Most Gram-negative bacteria synthesize osmo-regulated periplasmic glucans (OPG) in the periplasm or extracellular space. In this study, structural and functional analyses of OpgG and OpgD from Escherichia coli revealed that these proteins are β-1,2-glucanases with remarkably different activity from each other, establishing a new glycoside hydrolase family, GH186. Furthermore, a reaction mechanism with an unprecedentedly long proton transfer pathway among glycoside hydrolase families is proposed for OpgD. The conformation of the region that forms the reaction pathway differs noticeably between OpgG and OpgD, which explains the observed low activity of OpgG.

The D388N mutant was used to determine a Michaelis complex structure of EcOpgD because this mutant displayed the lowest activity among mutants of acidic amino acids conserved in its homologs, and this residue is located in the long cleft of the ligand-free structure. The complex structure was obtained as a dimer by co-crystallizing the D388N mutant with β-1,2-glucan. The substrate binding site is formed as a cleft in the ligand-free structure, whereas this site forms a tunnel in the structure of the complex. In EcOpgD, the seventh and eleventh Glc moieties from the reducing end of Sop13 form skew boat (1S3 and 1S5, respectively) conformations, according to the puckering coordinate system of a six-membered pyranose ring, Cremer–Pople parameters. A water molecule (Wat1) is located near the anomeric carbon of the seventh Glc moiety from the reducing end (3.5 Å). The angle formed by this water, the anomeric carbon and the glycosidic bond oxygen atom is 168.17°, which is close to 180° and suitable for the nucleophilic (in-line) attack of the anomeric carbon. The other Glc moiety with the skew boat conformation has no nucleophilic water because the O5 atom of the twelfth Glc moiety from the reducing end occupies the position for a nucleophile. These observations strongly suggest that the position of the seventh Glc moiety is subsite –1 and that EcOpgD accommodates a Sop13 molecule at subsites –7 to +6 as a Michaelis complex. D388 was identified as a general acid catalyst candidate because this acidic amino acid directly interacts with the oxygen atom of the glycosidic bond between subsites –1 and +1. No acidic residue directly interacting with the nucleophilic water is found in the complex structure, unlike canonical anomer inverting GH enzymes. Overall, a nucleophilic water is likely activated by D300 as a general base through the two water molecules (Wat2 and Wat3) and one substrate hydroxy group.

>[2x]MDRRRFIKGSMAMAAVCGTSGIASLFSQAAFAADSDIADGQTQRFDFSILQSMAHDLAQTAWRGAPRPLPDTLATMTPQAYNSIQYDAEKSLWHNVENRQLDAQFFHMGMGFRRRVRMFSVDPATHLAREIHFRPELFKYNDAGVDTKQLEGQSDLGFAGFRVFKAPELARRDVVSFLGASYFRAVDDTYQYGLSARGLAIDTYTDSKEEFPDFTAFWFDTVKPGATTFTVYALLDSASITGAYKFTIHCEKSQVIMDVENHLYARKDIKQLGIAPMTSMFSCGTNERRMCDTIHPQIHDSDRLSMWRGNGEWICRPLNNPQKLQFNAYTDNNPKGFGLLQLDRDFSHYQDIMGWYNKRPSLWVEPRNKWGKGTIGLMEIPTTGETLNNIVCFWQPEKAVKAGDEFAFQYRLYWSAQPPVHCPLARVMATRTGMGGFSEGWAPGEHYPEKWARRFAVDFVGGDLKAAAPKGIEPVITLSSGEAKQIEILYIEPIDGYRIQFDWYPTSDSTDPVDMRMYLRCQGDAISETWLYQYFPPAPDKRQYVDDRVMSLEHHHHHH>MRIPLVGKDSIESKDIGFTLIHEHLRVFSEAVRQQWPHLYNEDEEFRNAVNEVKRAMQFGVKTIVDPTVMGLGRDIRFMEKVVKATG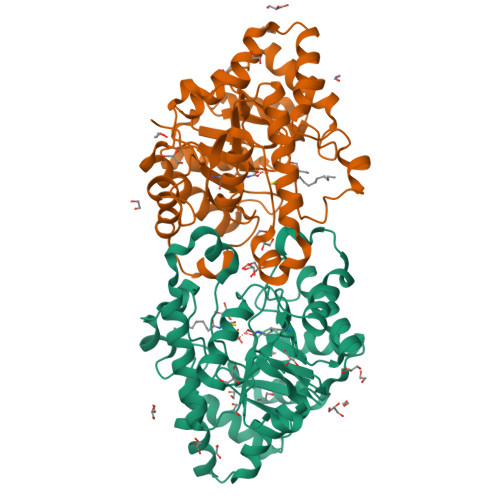INLVAGTGIYIYIDLPFYFLNRSIDEIADLFIHDIKEGIQGTLNKAGFVKIAADEPGITKDVEKVIRAAAIANKETKVPIITHSNAHNNTGLEQQRILTEEGVDPGKILIGHLGDTDNIDYIKKIADKGSFIGLDRYGLDLFLPVDKRNETTLRLIKDGYSDKIMISHDYCCTIDWGTAKPEYKPKLAPRWSITLIFEDTIPFLKRNGVNEEVIATIFKENPKKFFS[4x]> MDAYSTRPLTLSHGSLEHVLLVPTASFFIASQLQEQFNKILPEPTEGFAADDEPTTPAELVGKFLGYVSSLVEPSKVGQFDQVLNLCLTEFENCYLEGNDIHALAAKLLQENDTTLVKTKELIKNYITARIMAKRPFDKKSNSALFRAVGEGNAQLVAIFGGQGNTDDYFEELRDLYQTYHVLVGDLIKFSAETLSELIRTTLDAEKVFTQGLNILEWLENPSNTPDKDYLLSIPISCPLIGVIQLAHYVVTAKLLGFTPGELRSYLKGATGHSQGLVTAVAIAETDSWESFFVSVRKAITVLFFIGVRCYEAYPNTSLPPSILEDSLENNEGVPSPMLSISNLTQEQVQDYVNKTNSHLPAGKQVEISLVNGAKNLVVSGPPQSLYGLNLTLRKAKAPSGLDQSRIPFSERKLKFSNRFLPVASPFHSHLLVPASDLINKDLVKNNVSFNAKDIQIPVYDTFDGSDLRVLSGSISERIVDCIIRLPVKWETTTQFKATHILDFGPGGASGLGVLTHRNKDGTGVRVIVAGTLDINPDDDYGFKQEIFDVTSNGLKKNPNWLEEYHPKLIKNKSGKIFVETKFSKLIGRPPLLVPGMTPCTVSPDFVAATTNAGYTIELAGGGYFSAAGMTAAIDSVVSQIEKGSTFGINLIYVNPFMLQWGIPLIKELRSKGYPIQFLTIGAGVPSLEVASEYIETLGLKYLGLKPGSIDAISQVINIAKAHPNFPIALQWTGGRGGGHHSFEDAHTPMLQMYSKIRRHPNIMLIFGSGFGSADDTY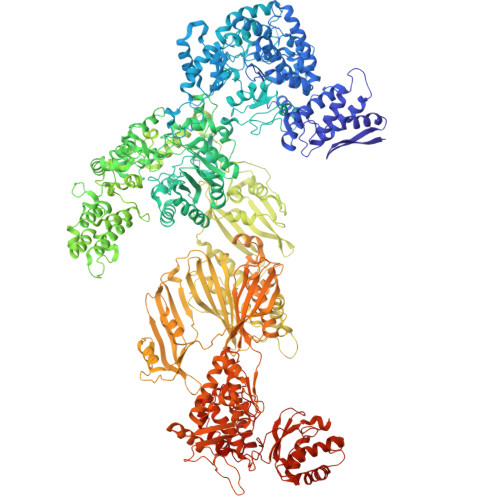PYLTGEWSTKFDYPPMPFDGFLFGSRVMIAKEVKTSPDAKKCIAACTGVPDDKWEQTYKKPTGGIVTVRSEMGEPIHKIATRGVMLWKEFDETIFNLPKNKLVPTLEAKRDYIISRLNADFQKPWFATVNGQARDLATMTYEEVAKRLVELMFIRSTNSWFDVTWRTFTGDFLRRVEERFTKSKTLSLIQSYSLLDKPDEAIEKVFNAYPAAREQFLNAQDIDHFLSMCQNPMQKPVPFVPVLDRRFEIFFKKDSLWQSEHLEAVVDQDVQRTCILHGPVAAQFTKVIDEPIKSIMDGIHDGHIKKLLHQYYGDDESKIPAVEYFGGESPVDVQSQVDSSSVSEDSAVFKATSSTDEESWFKALAGSEINWRHASFLCSFITQDKMFVSNPIRKVFKPSQGMVVEISNGNTSSKTVVTLSEPVQGELKPTVILKLLKENIIQMEMIENRTMDGKPVSLPLLYNFNPDNGFAPISEVMEDRNQRIKEMYWKLWIDEPFNLDFDPRDVIKGKDFEITAKEVYDFTHAVGNNCEDFVSRPDRTMLAPMDFAIVVGWRAIIKAIFPNTVDGDLLKLVHLSNGYKMIPGAKPLQVGDVVSTTAVIESVVNQPTGKIVDVVGTLSRNGKPVMEVTSSFFYRGNYTDFENTFQKTVEPVYQMHIKTSKDIAVLRSKEWFQLDDEDFDLLNKTLTFETETEVTFKNANIFSSVKCFGPIKVELPTKETVEIGIVDYEAGASHGNPVVDFLKRNGSTLEQKVNLENPIPIAVLDSYTPSTNEPYARVSGDLNPIHVSRHFASYANLPGTITHGMFSSASVRALIENWAADSVSSRVRGYTCQFVDMVLPNTALKTSIQHVGMINGRKLIKFETRNEDDVVVLTGEAEIEQPVTTFVFTGQGSQEQGMGMDLYKTSKAAQDVWNRADNHFKDTYGFSILDIVINNPVNLTIHFGGEKGKRIRENYSAMIFETIVDGKLKTEKIFKEINEHSTSYTFRSEKGLLSATQFTQPALTLMEKAAFEDLKSKGLIPADATFAGHSLGEYAALASLADVMSIESLVEVVFYRGMTMQVAVPRDELGRSNYGMIAINPGRVAASFSQEALQYVVERVGKRTGWLVEIVNYNVENQQYVAAGDLRALDTVTNVLNFIKLQKIDIIELQKSLSLEEVEGHLFEIIDEASKKSAVKPRPLKLERGFACIPLVGISVPFHSTYLMNGVKPFKSFLKKNIIKENVKVARLAGKYIPNLTAKPFQVTKEYFQDVYDLTGSEPIKEIIDNWEKYEQS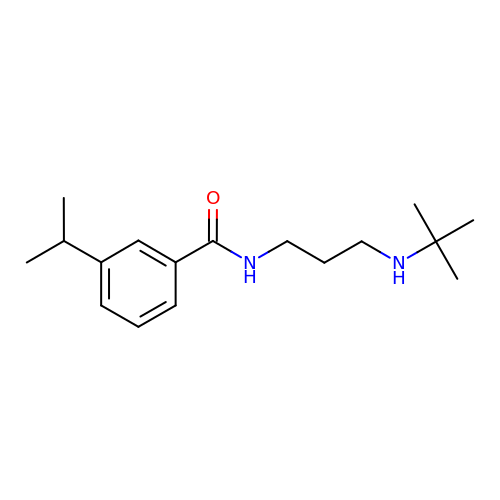N-[3-(tert-butylamino)propyl]-3-(propan-2-yl)benzamide | C17 H28 N2 O | CNTJLQUUYDXEFL-UHFFFAOYSA-N>[2x]GSHMRDVVSFEQPEFSVSRGDQVARIPVIRRVLDGGKSQVSYRTQDGTAQGNRDYIPVEGELLFQPGEAWKE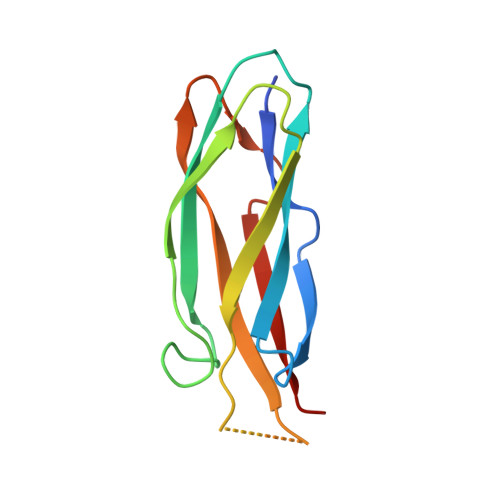LQVKLLELQEVDSLLRGRQVRRFHVQLSNPKFGAHLGQPHSTTIIIRDPDE>GAMGMLIENVEYDVLLERFKKILRQGGLKYTKQREVLLKTLYHSDTHYTPESLYMEIKQAEPDLNVGIATVYRTLNLLEEAEMVTSISFGSAGKKYELANKPHHDHMICKNCGKIIEFENPIIERQQALIAKEHGFKLTGHLMQLYGVCGDCNNQKAKVKI[2x]

One family, the ferric uptake regulator (Fur) family of metalloregulators, is involved in the regulation of iron, manganese, zinc and nickel homeostasis through the activity of Fur, Mur (manganese uptake regulator), Zur (zinc uptake regulator) and Nur (nickel uptake regulator) proteins, respectively. Previous structural studies of members of the Fur family of proteins revealed that these transcription factors fold into two distinct domains, including a DNA binding domain (DBD) and a dimerization domain (DD) localized on the N- and C-terminus of the protein, respectively. The third metal binding pocket is the regulatory site (S2) and is composed of residues located in a region referred to as the hinge, which links the DBD and DD. Gene regulation by CjFur occurs in both the presence and absence of regulatory metals.

To further understand the role of the S3 site in CjFur DNA binding activity, we carried out crystallization trials to solve the structure of the wild-type transcription factor devoid of metal in its S3 site. The structure shows that the protein assembles into a biological dimer in which each monomer folds into two domains, the DBD and the DD, reminiscent of other ferric uptake regulators. The modeled zinc atom is tetra-coordinated by C105, C108, C145 and C148 in the S1 metal binding site. Despite adopting a V-shape structure, no metals could be modeled in the S2 sites. Intriguingly, akin to the S2 site, no metals could be detected in the S3 site. Instead, four water molecules establish several hydrogen bonds with residues forming the S3 sites. The DBD of CjFurZn protomer A undergoes a clockwise rotation of ~5°, shifting the C-terminus of its α1-helix inwardly by ~5 Å. The DBD of CjFurZn protomer B does not undergo a rotation, but instead, its α3- and α4-helices are displaced toward the inner portion of the V-shaped cleft. Altogether, these observations show that the DBD can undergo asymmetric reorganization when the S3 site is not metalated. Altogether, these results show that while the loss of metal binding in the S3 site can be compensated by water molecules, it causes a distortion in the DBD that negatively affects DNA binding by CjFur.>[6x]MTLTMGFIGFGKSANRYHLPYLKTRNNIKVKTIFVRQINEELAAPYEERGVYFTTDLDELLNDKEIQVVTICTPAHTHYELAKKVILAGKSVIVEKPFCDTVEHAKELLALGREKGVVVMPYQNRRFDGDFLAVKQVVEQGFLGDIIEIESHIDYFRPGSITHEAPKEEGSFYSLGIHTMDRMISLFGRPNTVTYDIRNNEVEGAVDNYFDVGLHYGNQLK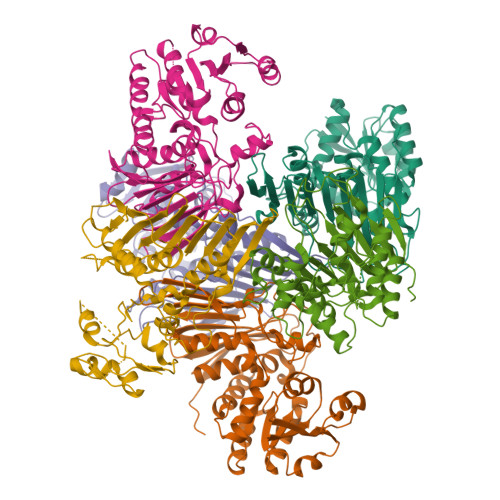IKLKTNHIVAKDYPRFIVHGTNGSFIKYGEDQQENDLKAGIMPESAGFGEDSPMYYGIAKYRNANGDWIEKQIKTPLGDYGRFYDAAYDTIVNGAPKLVKDEEAVTNIEILENGFAAPSPSVYKLEALHLNE>[2x]MIETITQS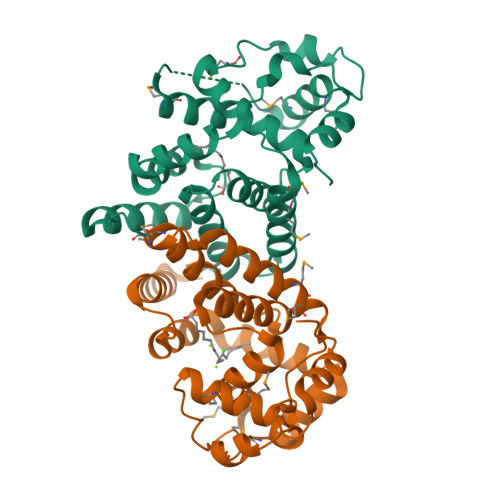QETAILESFLELVKSPYGNFASIGKLSHVLNDPDTLQKVVAVLSLTPQGKQAFEDRPMLGKIDLEQLHQLPNYTLGYMYADHMIRNQLTPPPVNENVNHPFMFLAAHLGETHDIWHVVTGCDTDKPGEVKLEAFYTAQLIPDRLFLALLAKNLLKTAMYEVELCEQILDGLTQGWMMGKRAKPLFGIEWNKLWETPLEELQTSLNIVPILEHHHHHH> MYRGFSLKLPNNYRSGQVTTEHRLPASNSHARWPVEVSFYSAVLHVPA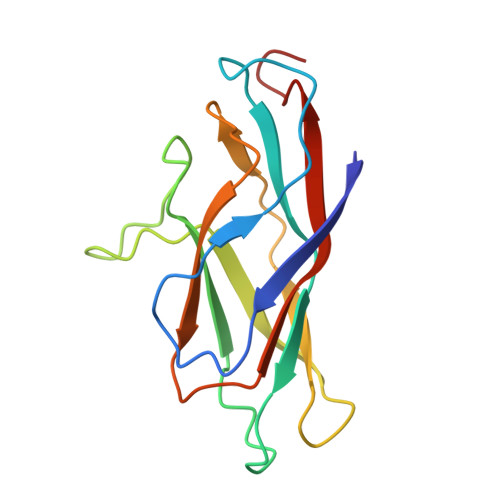KHQHKFPPVLELKLHNMTTGSMAAHRGSGHHFTFMFHAQSSPTEAVYSCVPVPIVFSDYQSNVIASVDMGEHDTAEKLHFYGSIRNCDNGCTY> MDSTKEKCDSYKDDLLLRMGLNDNKAGMEGLDKEKINKIIMEATKGSRFYGNELKKEKQVNQRIENMMQQKAQITSQQLRKAQLQVDRFAMELEQSRNLSNTIVHIDMDAFYAAVEMRDNPELKDKPIAVGSMSMLSTSNYHARRFGVRAAMPGFIAKRLCPQLIIVPPNFDKYRAVSKEVKEILADYDPNFMAMSLDEAYLNITKHLEERQNWPEDKRRYFIKMGSSVENDNPGKEVNKLSEHERSISPLLFEESPSDVQPPGDPFQVNFEEQNNPQILQNSVVFGTSAQEVVKEIRFRIEQKTTLTASAGIAPNTMLAKVCSDKNKPNGQYQILPNRQAVMDFIKDLPIRKVSGIGKVTEKMLKALGIITCTELYQQRALLSLLFSETSWHYFLHISLGLGSTHLTRDGERKSMSVERTFSEINKAEEQYSLCQELCSELAQDLQKERLKGRTVTIKLKNVNFEVKTRASTVSSVVSTAEEIFAIAKELLKTEIDADFPHPLRLRLMGVRISSFPNEEDRKHQQRSIIGFLQAGNQALSATECTLEKTDKDKFVKPLEMSHKKSFFDKKRSERKWSHQDTFKCEAVNKQSFQTSQPF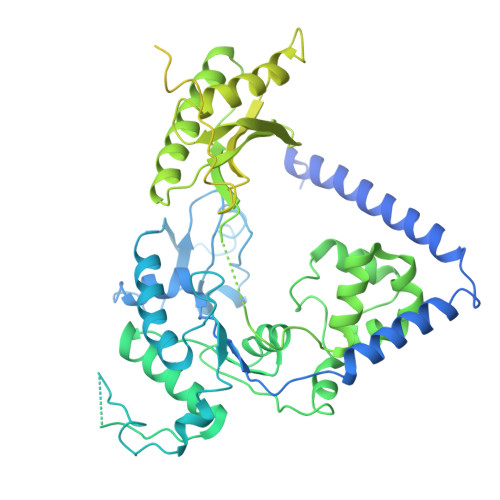QVLKKKMNENLEISENSDDCQILTCPVCFRAQGCISLEALNKHVDECLDGPSISENFKMFSCSHVSATKVNKKENVPASSLCEKQDYEAHPKIKEISSVDCIALVDTIDNSSKAESIDALSNKHSKEECSSLPSKSFNIEHCHQNSSSTVSLENEDVGSFRQEYRQPYLCEVKTGQALVCPVCNVEQKTSDLTLFNVHVDVCLNKSFIQELRKDKFNPVNQPKESSRSTGSSSGVQKAVTRTKRPGLMTKYSTSKKIKPNNPKHTLDIFFK1-(5-BROMO-PYRIDIN-2-YL)-3-[2-(6-FLUORO-2-HYDROXY-3-PROPIONYL-PHENYL)-CYCLOPROPYL]-UREA 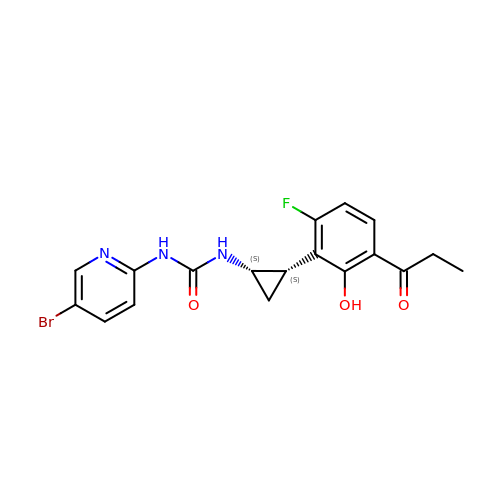| C18 H17 Br F N3 O3 | VRAJWAGCJIXJHQ-YPMHNXCESA-N(2R,3R,4S,5S)-5-amino-3,4-dihydroxytetrahydro-2H-pyran-2-yl 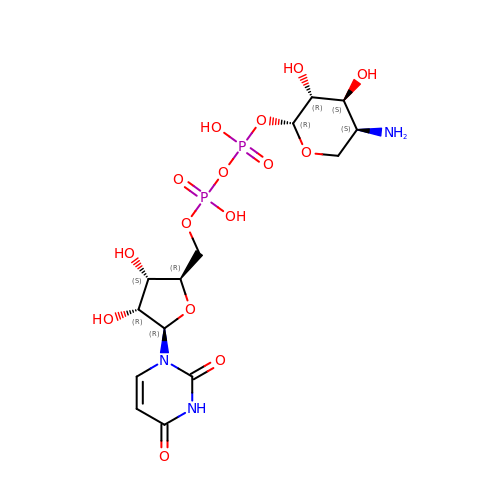[(2R,3S,4R,5R)-5-(2,4-dioxo-3,4-dihydropyrimidin-1(2H)-yl)-3,4-dihydroxytetrahydrofuran-2-yl]methyl dihydrogen diphosphate | C14 H23 N3 O15 P2 | GWBAKYBSWHQNMQ-IAZOVDBXSA-N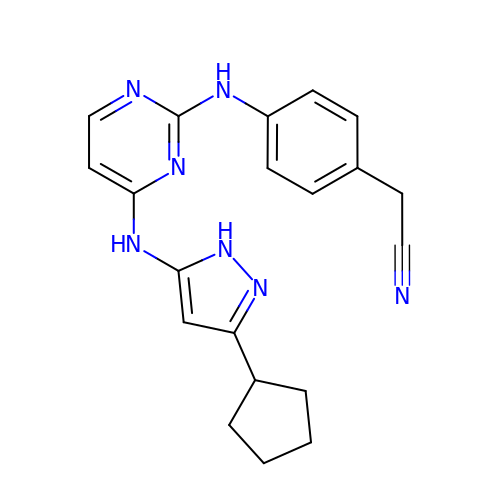[4-({4-[(3-cyclopentyl-1H-pyrazol-5-yl)amino]pyrimidin-2-yl}amino)phenyl]acetonitrile | C20 H21 N7 | VKAOLAKWGBXOCQ-UHFFFAOYSA-N>PKIVVVGAVAGGATCASQIRRLDKESDIIIFEKDRDMSFANCALPYVIGEVVEDRRYALAYTPEKFYDRKQITVKTYHEVIAINDERQTVSVLNRKTNEQFEESYDKLILSPGASANSLGFESDITFTLRNLEDTDAIDQFIKANQVDKVLVVGAGYVSLEVLENLYERGLHPTLIHRSDKINKLMDADMNQPILDELDKREIPYRLNEEINAINGNEITFKSGKVEHYDMIIEGVGTHPNSKFIESSNIKLDRKGFIPVNDKFETNVPNIYAIGDIATSHYRHVDLPASVPLAWGAHRAASIVAEQIAGNDTIEFKGFLGNNIVKFFDYTFASVGVKPNELKQFDYKMVEVTQGAHANFYPGNS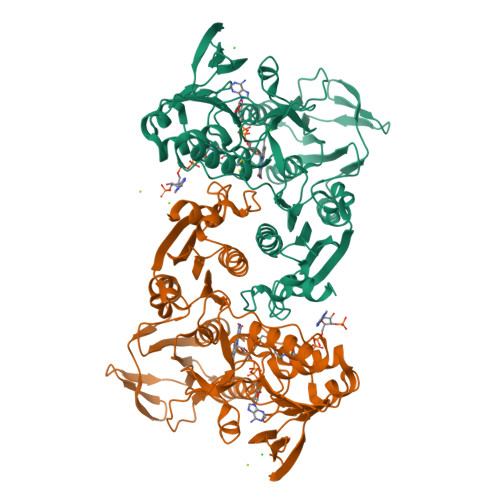PLHLRVYYDTSNRQILRAAAVGKEGADKRIDVLSMAMMNQLTVDELTEFEVAFAPPYSHPKDLINMIGYKAK[2x]>GSHMASMTGGQQMGRGSMTQDEMKKAAGWAALKYVEKGSIVGVGTGSTVNHFIDALGTMSEEIKGAVSSSVASTEKLEALGIKIFDCNEVASLDIYVDGADEINADREMIKGGGAALTREKIVAAIADKFICIVDGTKAVDVL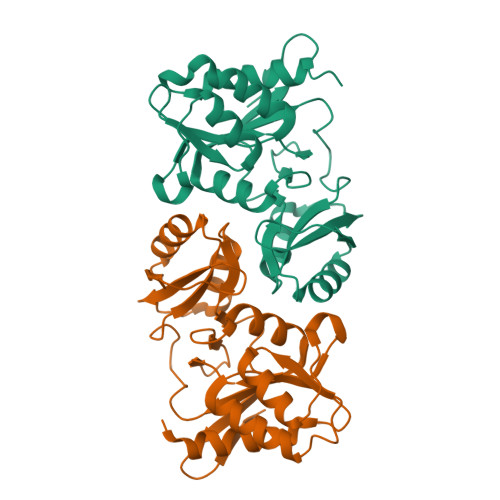GTFPLPVEVIPMARSYVARQLVKLGGDPCYREGVITDNGNVILDVYGMKITNPKQLEDQINAIPGVVTVGLFAHRGADVVITGTPEGAKIEE[2x]>MKHQHQHQHQHQHQQPLQEEEQAHATSLPPRASSPPQILPQLSPEQLGMIEKLVAAQQQCNRRSFSDRLRVTPWPMA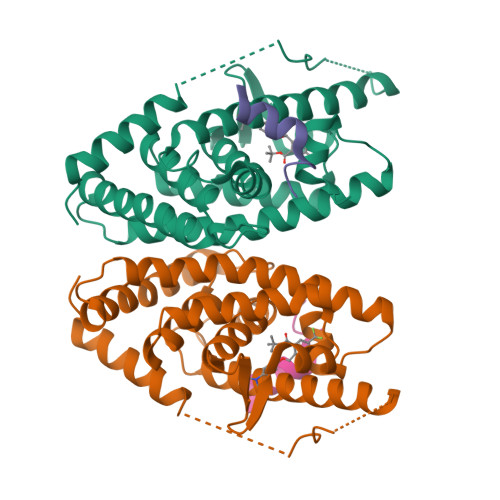PDPHSREARQQRFAHFTELAIVSVQEIVDFAKQLPGFLQLSREDQIALLKTSAIEVMLLETSRRYNPGSESITFLKDFSYNREDFAKAGLQVEFINPIFEFSRAMNELQLNDAEFALLIAISIFSADRPNVQDQLQVERLQHTYVEALHAYVSIHHPHDRLMFPRMLMKLVSLRTLSSVHSEQVFALRLQDKKLPPLLSEIWDVHE[2x];>[2x]CPSSHSSLTERHKILHRLLQEGSPS> SLDFSRNLYDIGEQLDSEDLASLKFLSLDYIPQRKQEPIKDALMLFQRLQEKRMLEESNLSFLKELLFRINRLDLLITYLNTRKEEMERELQTPGRAQISAYRVMLYQI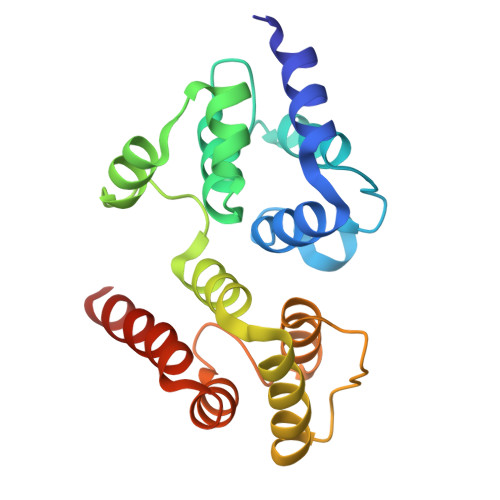SEEVSRSELRSFKALLQEEDSKCKLDDDMNLLDIFIEMEKRVILGEGKLDILKRVCAQINKSLLKIINDYEEFSKERSSS N-[(4S)-4-ammonio-4-carboxybutanoyl]-S-(4-bromobenzyl)-L-cysteinylglycine | 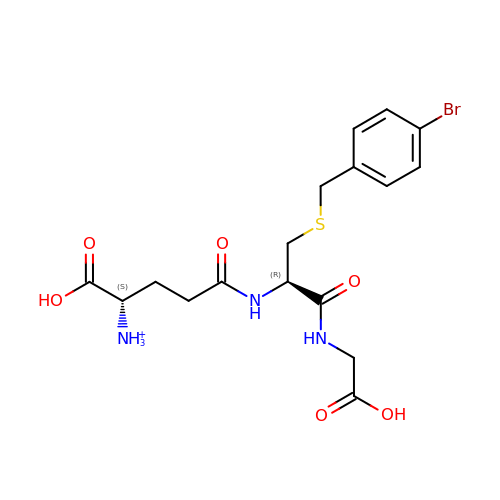C17 H23 Br N3 O6 S | HMNYAPVDRLKBJH-STQMWFEESA-O In the present study, we use cryoelectron microscopy to determine structures of the Desulfonema magnum (Dm) Craspase complex to gain mechanistic insights into its regulation. We used cryoelectron microscopy (cryo-EM) to analyze the Craspase complex, which resulted in two structures, one showing clear density for crRNA and all protein domains of the complex (DmCas7-11–crRNA and DmTPR-CHATfull), whereas the second lacks density for the regions of DmTPR-CHAT (DmCas7-11–crRNA and DmTPR-CHATNTD). DmTPR-CHAT makes multi-domain interactions with DmCas7-11–crRNA via its NTD and CTD, forming two major binding sites. The overall structure of D. magnum Craspase revealed that the complex adopts a ‘closed’ conformation characterized by the steric occlusion of the first segment of the spacer crRNA by the CLD.

DmTPR-CHAT organizes into three domains: the N-terminal domain (NTD), tetratricopeptide repeat (TPR) domain and the carboxy-terminal domain (CTD). The CTD contains a caspase-like subdomain (CLS) starting from β sheet-4 at its N terminus and terminating at β sheet-11 at its C terminus. The CLS is of particular interest because predictions suggest that it acts as a trigger for cell death or dormancy via a caspase-related peptidase activity. The CLS was also similar to Cas7 (± substrate) and PIGK (phosphotidylinositol glycan anchor biosynthesis class K) with the root mean square deviation (r.m.s.d.) between the C-α atoms of the protein backbones of 1.1 and 1.4 Å. The binding site of the NTD has a larger surface area than that of the CTD. At the other site, the CTD forms salt bridges with residues from the palms of Cas7.1 and Cas7.2. In contrast, the CLD in the Craspase complex stably associates with the complex, showing that DmTPR-CHAT promotes the rigidity of the CLD.

> MSSAFSGLKIPELSVDPAEVFKSDNPQLVSVLLDEFELQEQRPFFSGLIPEKQINIALKKSPQLKKLACHLLEAYEINGRRWKHADRRRVLEKAIRLLEKVSNELKGDIQKLENNVKESGKDSEELNKTREKHGEILADMGRAYLHRAKIIRPKGFTIPAKKKESLRKALDFCKEAKARHLAGLVGLEMDRCDMSDFDSENSLEKLLRDATTGVSLSKDQYYSNEYRKAEYYQMCIRLAEIEEDKHGATDEGSENNRYKRLEGILGPKKSQGKKKGKKNKKKKGTNSKSALEKIMAFEKFKVAVYLGEGKEKTHWNDFSEFLMRYPFSHPSWEDSVRFLRRLYKKGNDKWRELSVALWEIAKKNSAKTSSIHLRWYWSRQRDLYDLAFLSALEQADIAEDESVRQEKLRLAAKVADSAKNRPALTWQAMEQMADKDEALKKEIENYAQALGGGYIEQFEKTELPKNTNPQDDIPDDLKTSGLVVQFYLVHLKDYENGYALIYDGKTKKWSCEMFNFFPIWEKYLQWQSVYFDLPANQKEESADQLKALCLELGRHLYFLFDFEENRKAHEKNQDTAKENWDMLFIPHDFLHRVPIHGAIKKNGTNILLKKFNCTYFPTLPNASITPESPKSDNVAELIEYFSEHEKDYSEYFDKIEHIFDKKNRAATSQDLLDAAISPPRTLTIYCHGQSDVNNPFYSRLLLKDKLELIKLATLQEHYSGTHIFLGACETDLMPPLSAPLDEQLSMAAMFLQKGVGSVLGTLWEAYPRAVKDIVKNILSADDTQYFEKLFSLKKKISVNQKKSLYYYLCFKLYRSFDQIGKE;> MGSSHHHHHHSQDPMQHIIPLTITFLESFRVIEWHKSSDRNSLRFLRGYAYARWHRSLKNNKGRPYITGTLVRSAIIRAAEELLWLNDGNYKGAICCPGEFNGSNAKVFREGKARRLRRRQTLTWPTKCACHEKEPCPFCLLLGRYEKSSKTSKSPVLNNVNFSNFNVLGKEKEFLNIEDVADMRVVNRVDQQSGKAEDFFNIWEITDGAWKIFRGEIQVSDKGWSDEENFSKFLTLLKGASVLVDKISGGLCYLTLDKPELAELPAVKTEKDVLEPGDDASVLEISRPPYWNNMLNLAGTISEAFEREDKLVHLRLFADTVRELRRSDIETLDLPKGHADRLGKPSDHFIWDIEINKKVKLRNWLFWIFNEFRDTYAYFDWRTFCEALGQALYLEAKKQVPNQFSSERPVGATPAMEVKTPEHDPGRAAQGPRYEWLIKGELVSQTPFFFGWSTEADNREHTNLKLLAARDGRLRLPLSVLRGILRRDIKVVLDNKCRAELAMKQPCSCPVCNLMKKITIRDSFSSNYAEPPKIRHKIRLDPKSGTVAKGALFDSEVGPRGVVFPFELRLRSADDTLPQALKTVFSWWQQGTVSFSGDAGTGKGIFCLRNLKSIRWDLKTEMDKYAATLGGRKTPVGKWDKCHIPDDKTYPWVKETVEISVCSPFITKDPVNSLIDSAGYDAICYTTVDLEKSENINSLPESEISLLFEMFDLQYPMSYLFPNKDIYLLKGESFRGMLRTAVGRGENLLLREHEDCSCTLCRIFGNEHNAGKIRVEDFIIQGEPRTKLVDRVAIDRFTAGAKDKFKFDAAPIVGTPTNKLKFRGNIWIHRDLDGLACESLKLALEDIENGLYPFGGLGNAGFGWVNYNPLSHPAQEENKADFSLTKKMELNWSMKELSTDKIYWPHYFLPFGKKVLREKTPPSHACIDENEDSELYSGKIVCTLETRTPLIIPDSEFQGEEHKSYDFFNLNGELCIPGSEIRGMISSVFEALTNSCMRIFDEKKRLSWRMNPNKKDKKNNNRRELDDFIPGRVTNDRKMEEMKEYRYPFYDQAITANDKQNKYFDQWEATIELTDESLEKLKAEKILQSVLDALRPLTKKKEKYKNTETFVFDLKKFIGKIDDNQQMISEALERGKVRLTGNSLKQISKTKKIPRQILNQLKGLKDNTYENREQFISVLKTTVRGINDEQISLILDNIDEDVRLTDLSLTKIRKAKVPQTLVDMLADLKKDEPYKNEKEFLSEFKKKMGEIIGLILKHAAKTGGDVPRYNHPTPTDKMLLSLAAYNRNHKHENGKAEYRIVKPKHNLKVDFMFAVTPFENPFKGYNPAAVVEEPVGGYLKVSGPNKIEKVKKVNPNSVSVRDDKNQEIIHNGVYLRKITVANAKSKNKLRERLVPEFAWYDKDSEAAYAMTKRCERVFVEIGAKPIPIQPSAREKFKILTQEYQKNAKQQKTPEAFQTILPKDGELRPGDLVYFREDKKTNTVTDIIPVRISRTVDDEVLARKIPDDVGDVRPCVREILDKEKQKEIADAGVKEVFQHHPDGLCPACSLFGTTFYKGRIAFGFAFHKDKDPELANNGKHITLPLLERPRPTWSMPKKESRVPGRKFYVHHQGWERVIKHSNLDESDPNATKQTVNNRSVQAIKEEQKFQFEVRFENLREWELGLLVYVLQLEPQFAHKLGMGKALGFGSVRIRVGEIHSGPKELDESRLVSSAMKKMEEIWDRDKNVLEKLFRLLYFNESKDIKVRYPKLQKEKEEEEEESGYMELAKEEYQPEQRRNKLTNPWEGWGNILKKPAILI> DVYQEPTDPKFPQQWYLSGVTQRDLNVKAAWAQGYTGHGIVVSILDDGIEKNHPDLAGNYDPGASFDVNDQDPDPQPRYTQMNDNRHGTRCAGEVAAVANNGVCGVGVAYNARIGGVRMLDGEVTDAVEARSLGLNPNHIHIYSASWGPEDDGKTVDGPARLAEEAFFRGVSQGRGGLGSIFVWASGNGGREHDSCNCDGYTNSIYTLSISSATQFGNVPWYSEACSSTLATTYSSGNQNEKQIVTTDLRQKCTESHTGTSASAPLAAGIIALTLEANKNLTWRDMQHLVVQTSKPA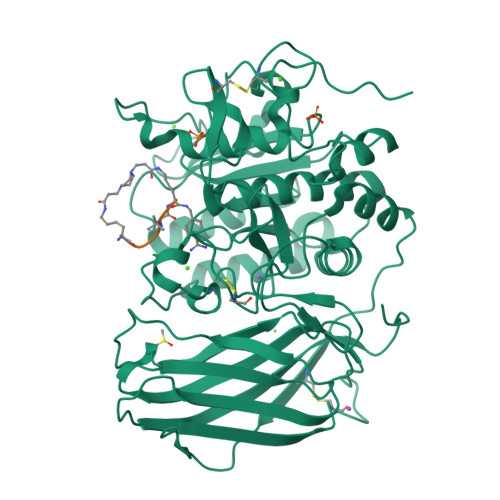HLNANDWATNGVGRKVSHSYGYGLLDAGAMVALAQNWTTVAPQRKCIIDILTEPKDIGKRLEVRKTVTACLGEPNHITRLEHAQARLTLSYNRRGDLAIHLVSPMGTRSTLLAARPHDYSADGFNDWAFMTTHSWDEDPSGEWVLEIENTSEANNYGTLTKFTLVLYGTASGSLVPRGSHHHHHH;> KRRVKX> MGSSHHHHHHSQDPAEKQKHDGRVKIGHYVLGDTLGVGTFGKVKIGEHQLTGHKVAVKILNRQKIRSLDVVGKIKREIQNLKLFRHPHIIKLYQVISTPTDFFMVMEYVSGGELFDYICKHGRVEEMEARRLFQQILSAVDYCHRHMVVHRDLKPENVLLDAHMNAKIADFGLSNMMSDGEFLRTSCGSPNYAAPEVISGRLYAGPEVDIWSCGVILYALLCGTLPFDDEHVPTLFKKIRGGVFYIPEYLNRSVATLLMHMLQVDPLKRATIKDIREHEWFKQGLPSYLFPEDPSYDANVIDDEAVKEVCEKFECTESEVMNSLYSGDPQDQLAVAYHLIIDNRRIMNQASEFYLASSPPSGSFMDDSAMHIPPGLKPHPERMPPLIADSPKARCPLDALNTTKPKSLAVKKAKWHLGIRSQSKPYDIMAEVYRAMKQLDFEWKVVNAYHLRVRRKNPVTGNYVKMSLQLYLVDNRSYLLDFKSIDDEVVEQRSGSSTPQRSCSAAGLHRPRSSFDSTTAESH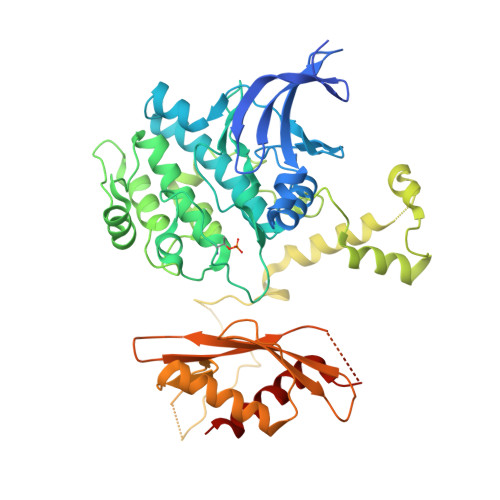SLSGSLTGSLTGSTLSSVSPRLGSHTMDFFEMCASLITTLAR> AQSVPWGISRVQAPAAHNRGLTGSGVKVAVLDTGISTHPDLNIRGGASFVPGEPSTQDGNGHGTHVAGTIAALNNSIGVLGVAPSAELYAVKVLGASGSGSVSSIAQGLEWAGNNGMHVANLSLGSPSPSAT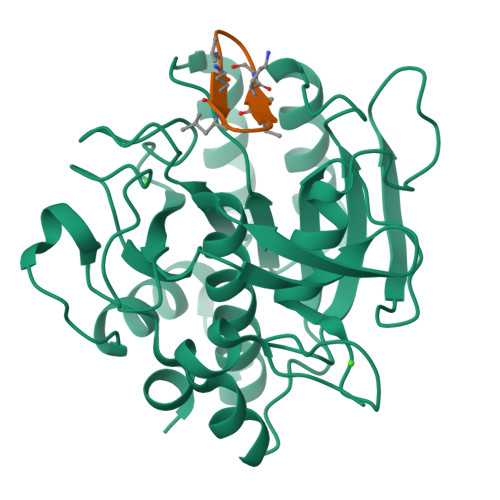LEQAVNSATSRGVLVVAASGNSGAGSISYPARYANAMAVGATDQNNNRASFSQYGAGLDIVAPGVNVQSTYPGSTYASLNGTSMATPHVAGAAALVKQKNPSWSNVQIRNHLKNTATSLGSTNLYGSGLVNAEAATR;> VALFPVALFP> AAKSYMSMTLSMPMGSARAGDGQDQANPDYHYVGEWAGKDKIEKVSIYMVPQGGPGLVESAEDLDFGTYYENPTIDPATHNAILKPKKGIKVNSAVGKTVKVYVVLNDIAGKAKALLANVNAADFDAKFKEIIELSTQAQALGTVADGPNPATAAGKIAKKNGTTDETIMMTCLQPSDALTIEAAVSEANAIAGIKNQAKVTVERSVARAMVSTKAQSYEIKATTQIGEIAAGSVLATITDIRWVVAQGERRQYLSKKRGTVPENTWVTPGSGFVPTSSTFHTNATEYYDYAGLWEDHNTNEAVISGTQVPTLADYQLQDVTGELANALSGKFLLPNTH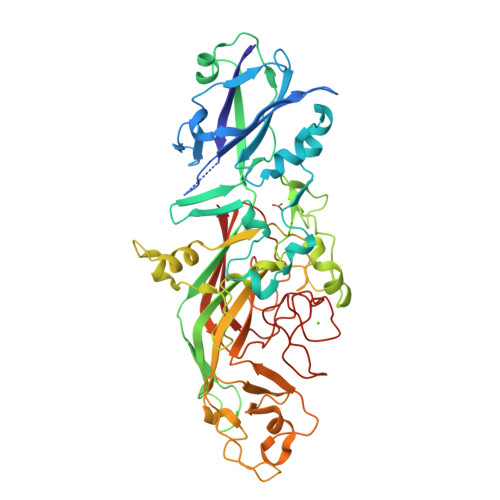KSGANAASSDYKRGNTAYVLVRAKFTPKKEAFIDRGKTYSDNTAVPEYVAGEDFFVGENGQFYVSMKSVTDPKVGGVAGMKAHKYVKGKVLYYAWLNPSTTSPDSWWNSPVVRNNIYHIHIKSIKKLGFNWNPLVPDPDPSNPENPNNPDPNPDEPGTPVPTDPENPLPDQDTFMSVEVTVLPW>[2x]MAAHHHHHHLAGIYLKVKGKTTGEIKGSVVQEGHDGKIHILAFKNDYDMPARLQEGLTPAAAARGTITLTKEMDRSSP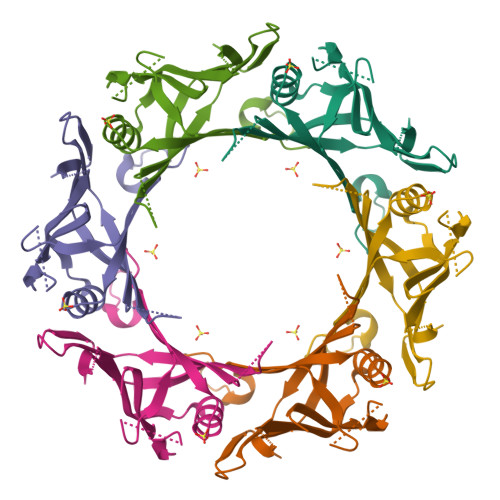QFLQALGKREMMEEFEITIYSPKADKETGGDLTELLFTYKFEKVLITHMDQYSPTPHKDDSNGIKEGLLGYIEEIKFTYSGYSLEHAESGIAGAANWKNG> VVGGEDAKPGQFPWQVVLNGK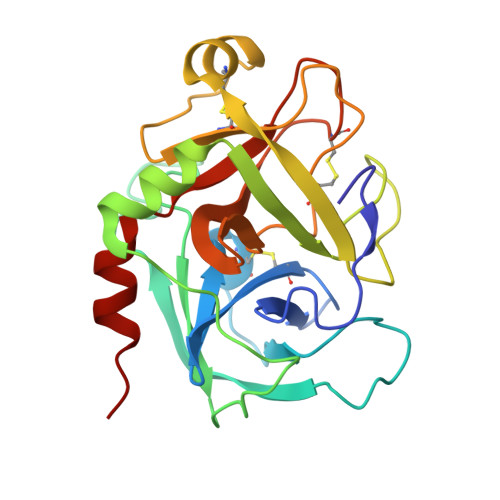VDAFCGGSIVNEKWIVTAAHCVETGVKITVVAGEHNIEETEHTEQKRNVIRIIPHHNYNAAINKYNHDIALLELDEPLVLNSYVTPICIADKEYTNIFLKFGSGYVSGWGRVFHKGRSALVLQYLRVPLVDRATCLRSTKFTIYNNMFCAGFHEGGRDSCQGDSGGPHVTEVEGTSFLTGIISWGEECAMKGKYGIYTKVSRYVNWIKEKTKLT We examined the crystal-packing interactions formed by the polo-box domain (PBD) of polo-like kinase 1 (Plk1), a validated anti-cancer target, whose phosphorylation-dependent protein–protein interactions are crucial for successful progression of the cell through mitosis. We have observed an unreported binding site in a number of crystal structures of the PBD, which is formed by the rearrangement of surface residues involved in crystal packing. This site is located close to the phosphopeptide-binding groove, making it potentially accessible for phosphorylated proteins binding to the PBD. The new binding site consists of seven residues: Val415, Leu478, and Phe482 form the bottom of the pocket whilst Tyr417, Tyr421, Tyr481, and Tyr485 form the sides of the pocket.

We further investigated the influence of Phe71PBIP1 on its interaction with the PBD. The thermal shifts of 9.7 °C observed for 72-DPPLHSpTA-79 (lacking Phe71), and 10.5 °C observed for 71-ADPPLHSpTA-79 were significantly lower than the one observed for 71-FDPPLHSpTA-79 and showed no significant difference between the wild-type and mutant protein. When DPPLHSpTA is bound to the protein, the hydrophobic pocket adopts a closed conformation and does not participate in peptide binding.

> GPLGSPEFDCHLSDMLQQLHSVNASKPSERGLVRQEEAEDPACIPIFWVSKWVDYSDKYGLGYQLCDNSVGVLFNDSTRLILYNDGDSLQYIERDGTESYLTVSSHPNSLMKKITLLKYFRNYMSEHLLKAGANITPREGDELARLPYLRTWFRTRSAIILHLSNGSVQINFFQDHTKLILCPLMAAVTYIDEKRDFRTYRLSLLEEYGCCKELASRLRYARTMVDKLLSSR;> XDPPLHSTAX Given the auxotrophic nature of pneumococci for certain amino acids, the Ami ABC transporter system, orchestrating oligopeptide uptake, becomes indispensable in host compartments lacking amino acids. The system comprises five exposed Oligopeptide Binding Proteins (OBPs) and four proteins building the ABC transporter channel. Crucially, SBPs determine the specificity of their respective transport systems, thereby governing the range of molecules capable of entering the cell. The five lipoproteins exhibit pairwise sequence identity of ~52–60% and share a very similar overall folding.

To mitigate uncertainties stemming from potential mixtures of different peptides in our crystallized structure, we conducted pre-incubation of the AmiA protein with an excess of synthetized peptide 5 before crystallization. This strategy facilitated the elucidation of the AmiA:peptide 5 complex at 1.76 Å resolution. Four independent monomers were found in the asymmetric unit, all with a highly similar structure (rmsd value ranging from 0.14 to 0.21 Å for 574 Cα atoms among the four monomers, using monomer B as a reference throughout the text). In this complex, the amine N-terminus of peptide 5 is stabilized in a manner analogous to the description provided above for the other complexes, involving pockets P1, P2 and P3 from the OBP. It forms a salt-bridge with an aspartic residue (D507) and engages in hydrophobic interactions with a neighboring tryptophan residue (W504). The initial four residues of the peptide (AKTI) establish antiparallel β-sheet-like interactions, engaging the terminal residues of the extended strand of β20 on one side and forming parallel β-sheet-like interactions with a loop of domain I (which includes residues S54 and N56, from pockets P2 and P3, respectively), on the opposite side. The oligopeptide adopts an extended conformation with minimal intramolecular interactions, displaying a kink of ~90° at residue 6, resulting in an “L” shape. The two isoleucine residues in peptide 5 (I4 and I6) tightly pack against each other, occupying the two hydrophobic pockets P4 (involving residues Y486 and V502) and P6 (formed by residues D443 [aliphatic chain], S446, Y449, F481 and L482), all situated in AmiA’s domain III. The lysine residue at position 2 (K2) of the oligopeptide is stabilized through a salt-bridge interaction with E524 and a H-bond with T528 (domain III, both residues located in P2) of AmiA. AmiA features an additional α helix in R1 (residues 523–530), a characteristic absent in AliB, AliC and AliD, which instead exhibit a four-residues-long 310 helix.

>[4x]ASSSSKSSDSSAPKAYGYVYTADPETLDYLISSKNSTTVVTSNGIDGLFTNDNYGNLAPAVAEDWEVSKDGLTYTYKIRKGVKWFTSDGEEYAEVTAKDFVNGLKHAADKKSEAMYLAENSVKGLADYLSGTSTDFSTVGVKAVDDYTLQYTLNQPEPFWNSKLTYSIFWPLNEEFETSKGSDFAKPTDPTSLLYNGPFLLKGLTAKSSVEFVKNEQYWDKENVHLDTINLAYYDGSDQESLERNFTSGAYSYARLYPTSSNYSKVAEEYKDNIYYTQSGSGIAGLGVNIDRQSYNYTSKTTDSEKVATKKALLNKDFRQALNFALDRSAYSAQINGKDGAALAVRNLFVKPDFVSAGEKTFGDLVAAQLPAYGDEWKGVNLADGQDGLFNADKAKAEFAKAKKALEADGVQFPIHLDVPVDQASKNYISRIQSFKQSVETVLGVENVVVDIQQMTSDEFLNITYYAANASSEDWDVSGGVSWGPDYQDPSTYLDILKTTSSETTKTYLGFDNPNSPSVVQVGLKEYDKLVDEAARETSDLNVRYEKYAAAQAWLTDSSLFIPAMASSGAAPVLSRIVPFTGASAQTGSKGSDVYFKYLKSQDKVVTKEEYEKAREKWLKEKAESNEKAQKELASHVK;>[4x]AKTIKITQTR Vertebrate type-IIa RPTPs comprise LAR, PTPσ and PTPδ, which share common domain architecture with a single transmembrane (TM) helix flanked by a large extracellular domain (ECD) and cytoplasmic tandem PTP domains: the membrane-proximal PTP domain (D1) is catalytically active, whereas the membrane-distal PTP domain (D2) is inactive. In mammals, presynaptic type-IIa RPTPs form trans-synaptic adhesion by specifically binding to their cognate postsynaptic organizers through their ECDs for inducing synaptic differentiation of neurons. To date, five different types of postsynaptic organizers for type-IIa RPTPs have been reported: interleukin-1 receptor (IL-1R) accessory protein (IL-1RAcP)7, IL-1RAcP-like-1 (IL1RAPL1)8, neurotrophin receptor tyrosine kinase C (TrkC), netrin-G ligand-3 (NGL-3)1011 and Slit- and Trk-like (Slitrk) family proteins. To elucidate the structural basis for decoding the ‘splice-insert signaling code' in the type-IIa RPTPs, we determined the crystal structures of PTPδ-ECD in complex with IL-1RAcP-ECD and IL1RAPL1-ECD.

The meB insertion of PTPδ is important for binding between PTPδ and IL1RAPL1. The lack of meB reduces the affinity fivefold. When the apo structure of PTPδ Ig1-Fn2 containing meA3 and lacking meB (PTPδA3B−), which we determined at 3.5 Å resolution, is superposed onto the IL1RAPL1-ECD-bound structure of PTPδ Ig1-Fn2 using the Ig1–Ig2 unit of PTPδ as the reference, the Ig3 domain of the apo PTPδA3B− is oriented in the opposite direction from that of the IL1RAPL1-ECD-bound PTPδ and cannot interact with IL1RAPL1, even if structural flexibility of the linker between the Ig2 and Ig3 domains of PTPδ is assumed. Therefore, the meB insertion likely acts as an adjustable linker to locate the Ig3 domain of PTPδ in the appropriate position for interacting with the Ig1 domain of IL1RAPL1, representing how the meB insertion contributes to the affinity between PTPδ and IL1RAPL1.

>[2x]ETPPRFTRTPVDQTGVSGGVASFICQATGDPRPKIVWNKKGKKVSNQRFEVIEFDDGSGSVLRIQPLRTPRDEAIYECVASNNVGEISVSTRLTVLREDQIPRGFPTIDMGPQLKVVERTRTATMLCAASGNPDPEITWFKDFLPVDTSNNNGRIKQLRSESIGALQIEQSEESDQGKYECVATNSAGTRYSAPANLYVRVRRVPPRFSIPPTNHEIMPGGSVNITCVAVGSPMPYVKWMLGAEDLTPEDDMPIGRNVLELNDVRQSANYTCVAMSTLGVIEAIAQITVKALPKPPGTPVVTESTATSITLTWDSGNPEPVSYYIIQHKPKNSEEPYKEIDGIATTRYSVAGLSPYSDYEFRVVAVNNIGRGPASEPVLTQTSEQAPSSAPRDVQARMLSSTTILVQWKEPEEPNGQIQGYRVYYTMDPTQHVNNWMKHNVADSQITTIGNLVPQKTYSVKVLAFTSIGDGPLSSDIQVITKHHHHHH> KLGDICFSLRYVPTAGKLTVVILEAKNLKKMDVGGLSDP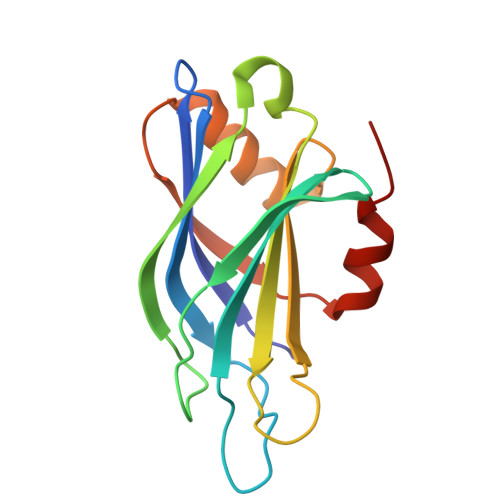YVKIHLMQNGKRLKKKKTTIKKNTLNPYYNESFSFEVPFEQIQKVQVVVTVLDYDKIGKNDAIGKVFVGYNSTGAELRHWSDMLANPRRPIAQWHTLQVEEEVDAMLAVKK>MAEQVALSRTQVCGILREELFQGDAFHQSDTHIFIIMGASGDLAKKKIYPTIWWLFRDGLLPENTFIVGYARSRLTVADIRKQSEPFFKATPEEKLKLEDFFARNSYVAGQYDDAASYQRLNSHMNALHLGSQANRLFYLALPPTVYEAVTKNIHESCMSQIGWNRIIVEKPFGRDLQSSDRLSNHISSLFREDQIYRINHYLGKEMVQNLMVLRFANRIFGPIWNRDNIACVILTFKEPFGTEGRGGYF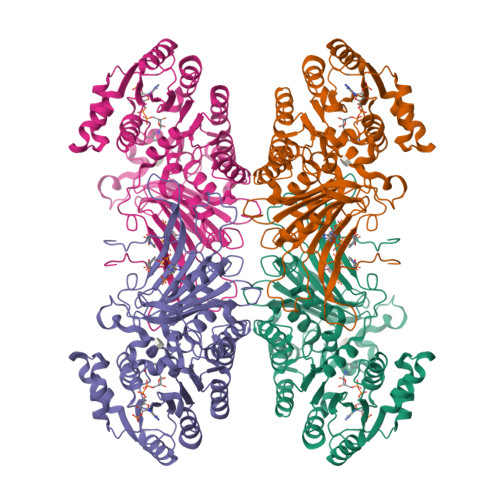DEFGIIRDVMQNHLLQMLCLVAMEKPASTNSDDVRDEKVKVLKCISEVQANNVVLGQYVGNPDGEGEATKGYLDDPTVPRGSTTATFAAVVLYVENERWDGVPFILRCGKALNERKAEVRLQFHDVAGDIFHQQCKRNELVIRVQPNEAVYTKMMTKKPGMFFNPEESELDLTYGNRYKNVKLPDAYERLILDVFCGSQMHFVRSDELREAWRIFTPLLHQIELEKPKPIPYIYGSRGPTEADELMKRVGFQYEGTYKWVNPHKLLEHHHHHH[4x]> MELIGDYSKAFLLQTVDGKHQDLKYISPETMVALLTGKFSNIVDKFVIVDCRYPYEYEGGHIKTAVNLP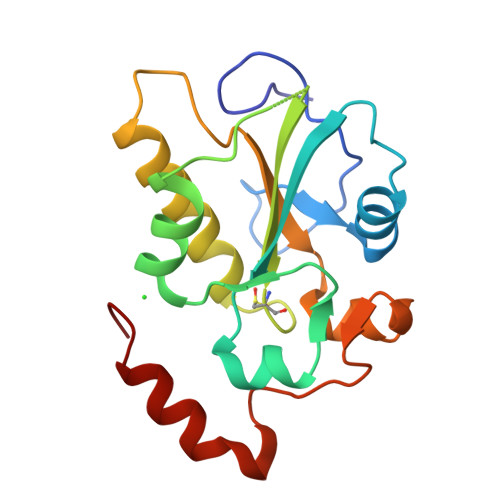LERDAESFLLKSPIAPCSLDKRVILIFHCEFSSERGPRMCRFIRERDRAVNDYPSLYYPEMYILKGGYKEFFPQHPNFCEPQDYRPMNHEAFKDELKTFRLKTRSW>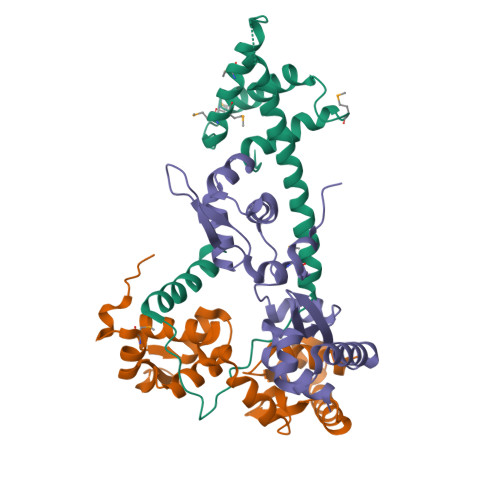 MDIKLKDFEGPLDLLLHLVSKYQMDIYDVPITEVIEQYLAYVSTLQAMRLEVTGEYMVMASQLMLIKSRKLLPKVAEVTDLGDDLEQDLLSQIEEYRKFKLLGEHLEAKHQERAQYYSKAPTELIYEDAELVHDKTTIDLFLAFSNILAKKKEEFAQNHT;>MSTLAKIEALLFVAGEDGIRVRQLAELLSLPPTGIQQSLGKLAQKYEKDPDSSLALIETSGAYRLVTKPQFAEILKEYSKAPINQSLSRAALETLSIIAYKQPITRIEIDAIRGVNSSGALAKLQAFDLIKEDGKKEVLGRPNLYVTTDYFLDYMGINHLEELPVIDELEIQAQESQLFGERI[2x]>MHHHHHHENLYFQGHMKKWGDMFTWGVSTSSYQIEGAANQGGRGPSIWDTFSKIPGAVANGDNGDVACDHYHRYNEDLDLMKWLGVGAYHFSIAWPRVIPSGYGALNKEGMDFYDRLIDGALERGITPWPTLYHWDLPQSLQDKGGWNNRDCAYWFAEYSQKMAEAFSDRLKNWITINEPFCSAWLGHLYGVMAPGIKDLKTGINASHHLLLGHGLATKAIREVSSELKVGITLNFTPAITLGESSEDKLAVELADGFDNRWFGDPVFKAKYPEDIVKAFGKEVPIHPGDMEIISTPLDYLGLNYYFRQTVEYDATAKPLPYKQVTAPNVERTGMGWEVHAQSF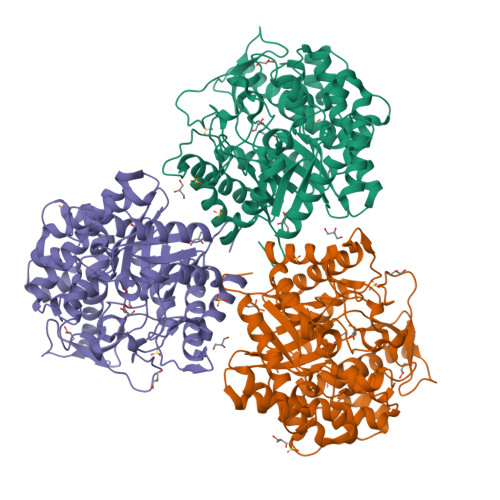TELLERVSKEYKPKEIFITENGSAWDDEVVDGKVDDPNRVSYLERHLDAMFAAKNKGVPISGYFAWSLIDNFEWAYGYAKRFGIIYVDYQTQKRIPKSSAYYYQKRIKESG[3x]> LPSYVDWRSAGAVVDIKSQGECGGCWAFSAIATVEGINKIVTGVLISLSEQELIDCGRTQNTRGCNGGYITDGFQFIINNGGINTEENYPYTAQ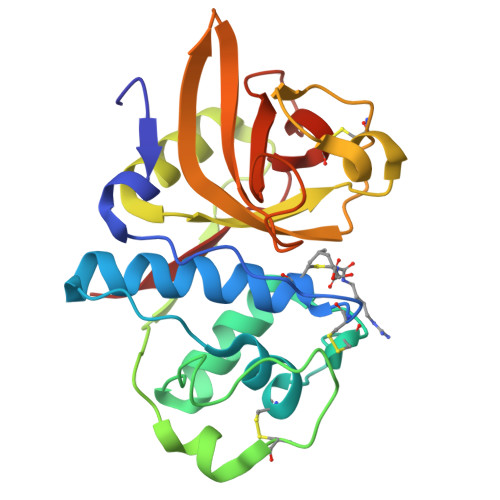DGECNVDLQNEKYVTIDTYENVPYNNEWALQTAVTYQPVSVALDAAGDAFKQYSSGIFTGPCGTAIDHAVTIVGYGTEGGIDYWIVKNSWDTTWGEEGYMRILRNVGGAGTCGIATMPSYPVKY> MAHHHHHHMVLNYFYPGTKTLKNKLGIMGYKQLEKRCKRNAKKVINSLRNEPLPETFDSSYLKYLHKRLFGSAFEWAGYTRDLSFAFDDGTIA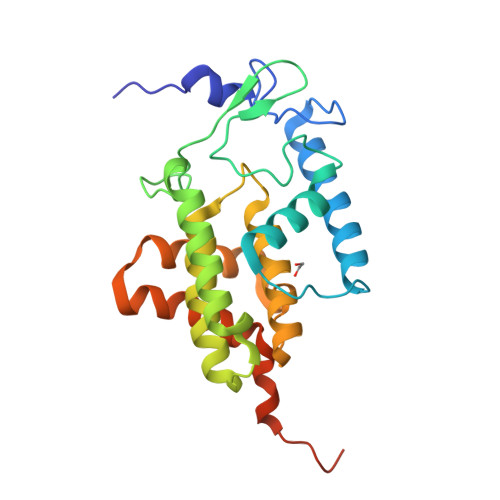QMSMMKIPGTDIYFAHGDKIQENLKEFDEILASKSNLQGLSREDFIEETVKLFSFLNYIHPFRAGNEAVQHIFFEKLAEAAGHKLDFSVVTEERIMRACNDAMALKGEEAHQAMKSLFEDISNPEEVIILRDFFKHIPRVERQRLNDE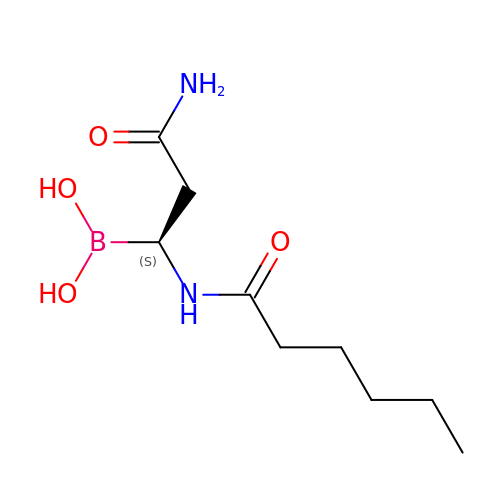[(1S)-3-amino-1-(hexanoylamino)-3-oxopropyl]boronic acid | C9 H19 B N2 O4 | JFQHYAGISMLDGO-SSDOTTSWSA-N4-[[3-chloro-4-(1-methylimidazol-2-yl)sulfanyl-phenyl]amino]-7-[3-(2-hydroxyethyl-methyl-amino)propoxy]-6-methoxy-quinoline-3-carbonitrile 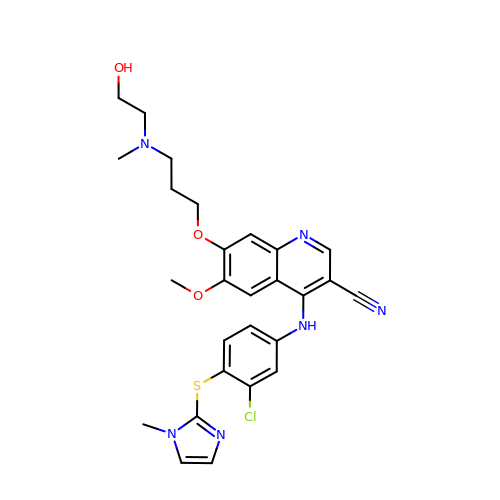| C27 H29 Cl N6 O3 S | QEMHSTOIAUCOQF-UHFFFAOYSA-N>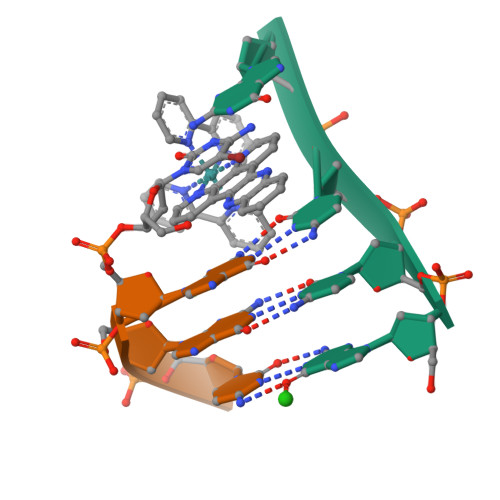 GCCG>QSVISANEIMDLLRGMDARLQHLEQKVDK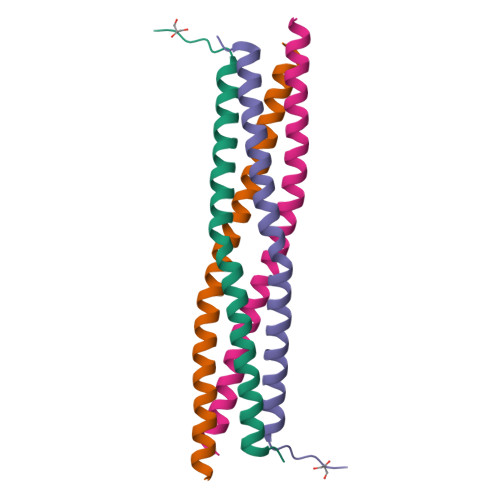VLAQGSMVTQIKNELSTVKTTLATIEGMMATVKIMD[2x]Mammalian target of rapamycin complex 1 (mTORC1) serves as a central regulator of cell growth and proliferation by integrating signals from growth factors, nutrients, energy status, and cellular stress. A small GTPase, called Ras homolog enriched in brain (Rheb), is a positive regulator of mTORC1. Like other small GTPases, the function of Rheb is dictated by its guanine nucleotide binding states: it is active in the GTP-bound form and inactive in the GDP-bound form. The Y35N mutant assumes a very similar overall structure as the WT Rheb with a typical small GTPase protein fold composed of a six-stranded β-sheet surrounded by four α-helices.

Surprisingly, the Y35N mutant, which was initially identified in several human cancers (Lawrence et al., 2014), could significantly increase the phosphorylation level of mTORC1 substrate S6K1 compared to the wild-type (WT) Rheb, and thus is regarded as a constitutively active mutant (Grabiner et al., 2014; Heard et al., 2014). To investigate the molecular basis for the constitutive activation of mTORC1 by the Y35N mutant, we determined the crystal structures of Y35NGppNHp and Y35NGDP at 2.0 Å and 2.1 Å resolution, respectively. On the other hand, the overall structure of Y35NGDP is more similar to that of WTGppNHp (RMSD of 0.79 Å for 162 Cα atoms) than that of WTGDP (RMSD of 0.92 Å for 162 Cα atoms) or Y35AGDP (RMSD of 0.97 Å for 167 Cα atoms). In the Y35NGDP structure, no Mg2+ could be identified at the active site, although Mg2+ is present in the protein storage buffer and the crystallization solution. In contrast, the switch I region and the binding mode of GDP exhibit notable difference in Y35NGDP and WTGDP (RMSD of 2.2 Å for 9 Cα atoms of the switch I region using the least-squares fitting method). Similarly, in Y35AGDP, the switch I region adopts a similar conformation as that in WTGDP, suggesting that mutation Y35A does not affect the conformation of switch I. However, in Y35NGDP, the side chain of Asn35 flips away from the nucleotide and points toward the solvent (about 180° rotation from that of Asn35 in Y35NGppNHp). Meanwhile, the side chain of Thr38 extends slightly closer toward the nucleotide, and thus occupies in part the position of Mg2+ and forms a hydrogen bond with the β-phosphate of GDP. In the Y35NGDP structure, the switch I region assumes a similar conformation as WTGppNHp and Y35NGppNHp and, in particular, the side chain of Thr38 is oriented toward the nucleotide to avoid steric conflict with mTOR, and hence both Pro37 and Ile39 are in proper positions to make tight interactions with mTOR. In other words, Y35NGDP mimics WTGppNHP in binding to mTOR and thus is capable to activate mTORC1 in a similar way as WTGppNHp.

>MPQSKSRKIAILGYRSVGKSSLTIQFVEGQFVDSNDPTIENTFTKLITVNGQEYHLQLVDTAGQDEYSIFPQTYSIDINGYILVYSVTSIKSFEVIKVIHGKLLDMVGKVQIPIMLVGNKKDLHMERVISYEEGKALAESWNAAFLESSAKENQTAVDVFRRIILEAEKLEHHHHHH[4x]> ATQGVFTLPANTRFGVTAFANSSGTQTVNVLVNNETAATFSGQSTN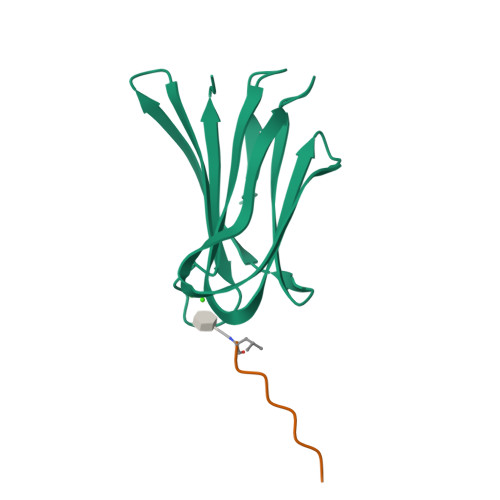NAVIGTQVLNSGSSGKVQVQVSVNGRPSDLVSAQVILTNELNFALVGSEDGTDNDYNDAVVVINWPLG;> LKALKKLA>GAASMKIINTTRLPEALGPYSHATVVNGMVYTSGQIPLNVDGKIVSADVQAQTKQVLENLKVVLEEAGSDLNSVAKATIFIKDMNDFQKINEVYGQYFNEHKPARSCVEVARLPKD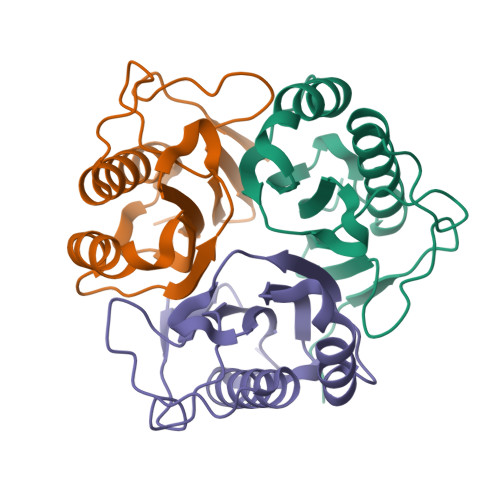VKVEIELVSKIKEL[6x]> MADTQYILPNDIGVSSLDSREAFRLLSPTERLYAYHLSRAAWYGGLAVLLQTSPEA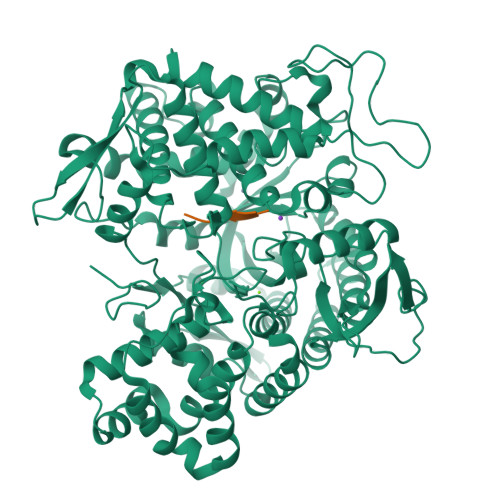PYIYALLSRLFRAQDPDQLRQHALAEGLTEEEYQAFLVYAAGVYSNMGNYKSFGDTKFVPNLPKEKLERVILGSEAAQQHPEEVRGLWQTCGELMFSLEPRLRHLGLGKEGITTYFSGNCTMEDAKLAQDFLDSQNLSAYNTRLFKEVDGCGKPYYEVRLASVLGSEPSLDSEVTSKLKSYEFRGSPFQVTRGDYAPILQKVVEQLEKAKAYAANSHQGQMLAQYIESFTQGSIEAHKRGSRFWIQDKGPIVESYIGFIESYRDPFGSRGEFEGFVAVVNKAMSAKFERLVASAEQLLKELPWPPTFEKDKFLTPDFTSLDVLTFAGSGIPAGINIPNYDDLRQTEGFKNVSLGNVLAVAYATQREKLTFLEEDDKDLYILWKGPSFDVQVGLHALLGHGSGKLFVQDEKGAFNFDQETVINPETGEQIQSWYRCGETWDSKFSTIASSYEECRAESVGLYLSLHPQVLEIFGFEGADAEDVIYVNWLNMVRAGLLALEFYTPEAFNWRQAHMQARFVILRVLLEAGEGLVTITPTTGSDGRPDARVRLDRSKIRSVGKPALERFLRRLQVLKSTGDVAGGRALYEGYATVTDAPPESFLTLRDTVLLRKESRKLIVQPNTRLEGSDVQLLEYEASAAGLIRSFSERFPEDGPELEEILTQLATADARFW;> YGGFL> MTTMSTATARPEATLPPGTPVITGWSAVSPYGIGRAEFAAGVRAGAKTAVKADAGLGPLPSSDVCTVPGFDIQEQLGPRGTAKMDRLTALALVASDGLLLDADGNRAVATDELTGVVLGITMGS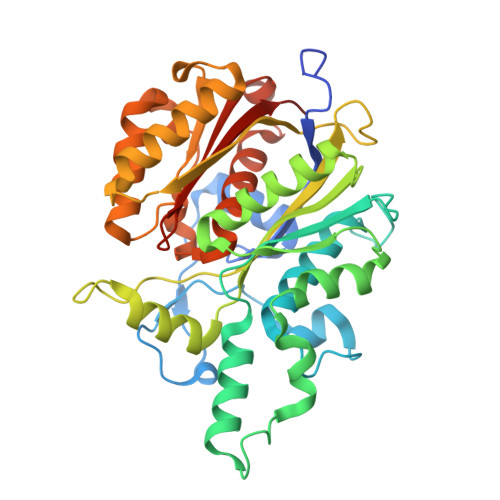LENVTDFLRQSYTNARPFYVDAGRIPFGSLNHAAGATAIRHDLKGPNTTVAGGRVSGLLALNYARRLMGQGRATKYLVGSAEEFSAAHAWFEHTATASGDPAPLLGEGCGLFLVEQAEAAERPPLAAVLSVETRVDIDDDPGAAVTACARRALRRAGVDAGEVWAAVPCAAPTAAGRAEHEALAALVPADALSRVPSMELLGDTGAASASFQIAAVLAAAEADADSRGRIALVCAVDRDGAVAVAVLRLIGEQR3-naphthalen-1-yl-~{N}-oxidanyl-propanamide | C13 H13 N O2 | 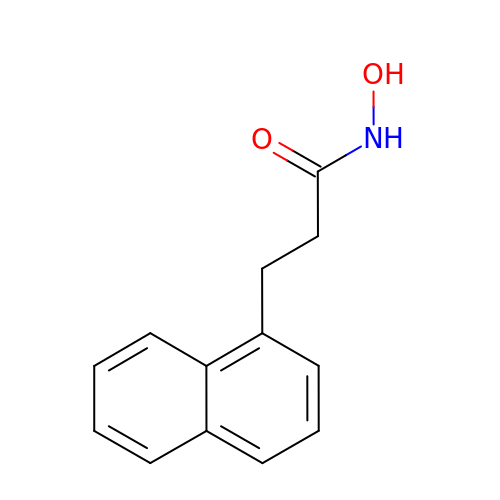ISLPNEHHRRPVDH-UHFFFAOYSA-N>TTLSTKQKQFLKGLAHHLNPVVMLGGNGLTEGVLAEIENALNHHELIKVK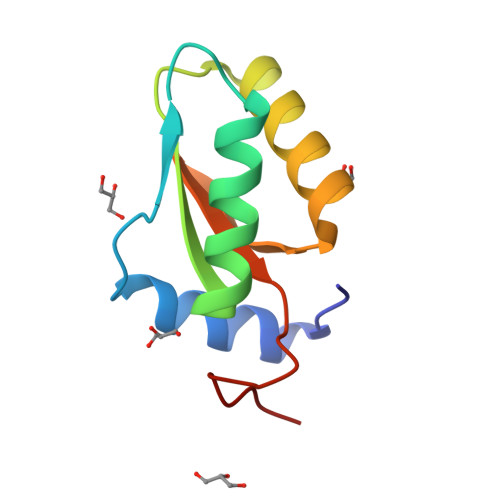VAGADRETKQLIINAIVRETKAAQVQTIGHILVLYRPSEEAKIQLPRK[2x]MukBEF folds the chromosome of Escherichia coli and related bacteria. The SMC protein MukB dimerizes at its ‘‘hinge’’ domain, which connects via the long coiled-coil ‘‘arm’’ to the ABC-type ATPase ‘‘head’’ domain. The heads are bridged by the kleisin MukF, whereby the C-terminal winged-helix domain (cWHD) of MukF binds the ‘‘cap’’ surface of one MukB, and the N-terminal middle domain (MD) binds the coiled-coil ‘‘neck’’ of the other MukB. MukF also recruits the dimeric KITE protein MukE.

In addition to a sample under ATP turnover conditions, we collected datasets where sodium vanadate or beryllium fluoride had been added 1 h after reaction start. These compounds poison the ATPase by replacing the released gamma-phosphate and can be used to enrich for species with engaged ATPase heads. All three conditions enabled the reconstruction of a state with engaged heads, and we pooled the datasets to increase the signal and obtain higher resolution (STAR Methods). At the resolution limits of ~3.5 Å, the nucleotide density was indistinguishable between samples and was modeled as ATP (STAR Methods). The resolved state was free of DNA, and the neck gate had opened widely. ATP binding and head engagement had triggered the detachment of the MukF MD from the MukB neck, which resulted in a swing-out of the MD of about 180°. Detachment of the MD was facilitated by the mechanical distortion of the MukB neck constrained between engaged heads and aligned arms, while the MD swing-out was stabilized by the binding of MukE to the top surface of the heads. Our structure reveals that occupation of the top of the heads by MukE and DNA is mutually exclusive, suggesting that MukE senses the DNA-free state of the heads to open the neck gate. ATP binding induces engagement of the heads within a MukBEF monomer, enabling ATP hydrolysis and subsequent head disengagement.

>[2x]MIERGKFRSLTLVNWNGFFARTFDLDELVTTLSGGNGAGKSTTMAAFVTALIPDLTLLHFRNTTEAGATSGSRDKGLHGKLRAGVCYSTLDVINSRHQRVVVGVRLQQVAGRDRKVDIKPFMIQGLPTAIQPTQLLTENVGERQARVLPLNELKDRLDEMEGVQFKQFNSITDYHAQMFDLGVIPKRLRSASDRSKFYRLIEASLYGGISSAITRSLRDYLLPENSGVRKAFQDMEAALRENRITLEAIRVTQSDRDLFKHLITEATSYVSADYMRHANERRTHLDEALALRGELFGSHKQLATEQYRHVEMARELAEQSGASSDLETDHQAASDHLNLVQTAMRQQEKIDRYQVDLEELSYRLEEQTDVVEEAGELQAEYEARTEATEQEVDELKSQLADYQQALDVQQTRAIQYQQALQALERARELCRLPDLSVDNAEEWLETFQAKEQQATEALLALEQKLSVADAAHNQFEQAYQLVKNIVGETSRSEAWQSARELLRDWPSQRHLADRVQPLRMRLSELEQRLNNQQNAERLLSEFCKRQGRQYQAEDLEALQNELEARQEALSLSVNEGGERRMEMRQELEQLKQKIQSLTARAPVWLAAQDTLNQLCEQSGETLASSNDVTEYMQQLLEREREATVERDEVAAQKRELEKQIERLSQPSGAEDSRMIALAERFGGVLLSEIYDDITIDDAPYFSALYGPARHGIVVPDLSLVRPHLETLEDCPEDLYLIEGDPQSFDDSVFNAEEQTNAVLVKSSDRQWRYSRYPELPLFGRAARENRLEALNLERDALAERYATLSFDVQKIQRAHQAFSQFVGKHLSVAFDTDPEAEIRELRQRHTELEREVSRFEDQTQQQRQQYAQAKESLTTLNRLIPQVTLLLDETLIDRVEEVREEMDEAQEAARFLQQHGSALTKLEPMVAVLQSDPQQHEQLQQDYETAKHSQHQAKQQAFALVEIVQRRVHFSYSDSAGMLSENADLNDKLRQRLEHAESDRSRAREQLRQQQAQYSQFNQVLASLKSSYETKQDMLKELLQEMKDIGVQADANAEMRARERRDRLHEALSVNRSRVNQLEKQIAFCEAEMENVQKKLRKLERDYYQIREQVVSAKAGWCAVMRMVKDNGVERRLHRRELAYMEGGALRSMSDKALGALRLAVADNEHLRDALRLSEDPKRPERKVQFFIAVYQHLRERIRQDIIRTDDPVDAIEQMEIELARLTEELTAREQKLAISSKSVANIIRKTIQREQNRIRMLNQGLQAVSFGQVRGVRLNVNVRESHAILLDVLSEQQEQHQDLFNSQRLTFSEAMAKLYQRLNPQVDMGQRLPQTIGEELLDYRNYLELDVEVNRGSDGWLKAESGALSTGEAIGTGMSILVMVVQSWEEESRRLRGKDISPCRLLFLDEAARLDAKSIATLFELCERLQMQLIIAAPENISPEKGTTYKLVRKVFKNHEHVHVVGLRGFGQDAPATQLISDVTA;>[2x]MSEYSQTVPELVSWARKNDFSISLPVERLAFLMAIAVLNSERLDGEMSEGELIDAFREVCKGFEQTAESVAVRANNAINDMVRQKLLNRFTSELADGNAIYRLTPLGISISDYYIRQREFSTLRLSMQLSIVANELHRAAEAAEEGGDEFHWHRNVFAPLKYSVAEIFDSIDMSQRLMDEQQNFVKEDIAALLNQDWQAAIANCEQLLSETSGTLRELQDTLEAAGDKLQANLLRIQDANMGSGGSELVDKLVFDLQSKLDRIISWGQQAIDLWIGYDRHVHKFIRTAIDMDKNRIFSQRLRQSVQHYFDNPWTLTVANAERLLDMRDEELALRNEEVTGELPLELEYEEFSEINDQLAAMIEKALLVYQQEQRPLDLGAVLRDYLAQHPLPRHFDVARILVDQAVRLGVAEADFSGLPAEWLAINDYGAKVQAHVIDTY;>MSSTHIEQFMPVKLAQALANSLFPELDSQLRAGRHIGIDDLDNHAFLMDFQEQLEEFYARYNVELIRAPEGFFYLRPRSTTLIPRSVLSELDMMVGKILCYLYLSPERLANQGIFTSQELYEELISLADEGKLMKFVNQRSSGSDLDKQKLQEKVRTTLNRLRRLGMVYFLPNNNNKFTITEAVFRFGADVRSGDDPREIQLRMIRDGEAMPVEGSLSLDDSENDETPDNSAEGAGDEQP[2x];>MSTIEERVKKIIGEQLGVKQEEVTNNASFVEDLGADXLDTVELVMALEEEFDTEIPDEEAEKITTVQAAIDYINGHQA[2x]>MAKSYKSVALVVGVTG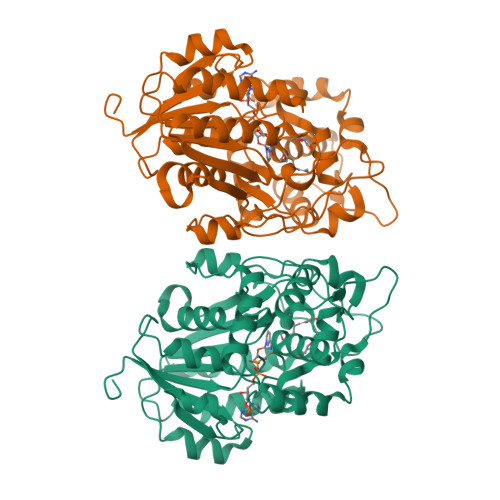IVGSSLAEVLKLPDTPGGPWKVYGVARRPCPVWLAKKPVEYIQCDVSDNQETISKLSPLKDITHIFYVSWIGSEDCQTNATMFKNILNSVIPNASNLQHVCLQTGIKHYFGIFEEGSKVVPHDSPFTEDLPRLNVPNFYHDLEDILYEETGKNNLTWSVHRPALVFGFSPCSMMNIVSTLCVYATICKHENKALVYPGSKNSWNCYADAVDADLVAEHEIWAAVDPKAKNQVLNCNNGDVFKWKHIWKKLAEEFGIEMVGYVEGKEQVSLAELMKDKDQVWDEIVKKNNLVPTKLKEIAAFWFADIAFCSENLISSMNKSKELGFLGFRNSMKSFVSCIDKMRDYRFIP[4x]> MSLEGGRRARVVIESKRNFFLGAFPTPFPAEHVELGRLGDSETAMVPGKGGADYILLPFKKMDFSRNLYDIGEQLDSEDLA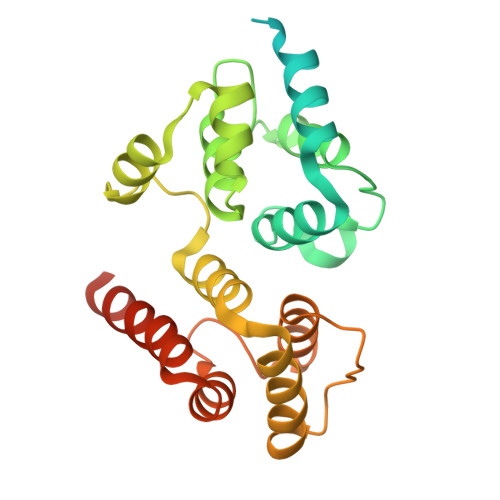SLKFLSLDYIPQRKQEPIKDALMLFQRLQEKRMLEESNLSFLKELLFRINRLDLLITYLNTRKEEMERELQTPGRAQISAYRVMLYQISEEVSRSELRSFKALLQEEDSKCKLDDDMNLLDIFIEMEKRVILGEGKLDILKRVCAQINKSLLKIINDYEEFSKERSSSEGHHHHHH> MTAI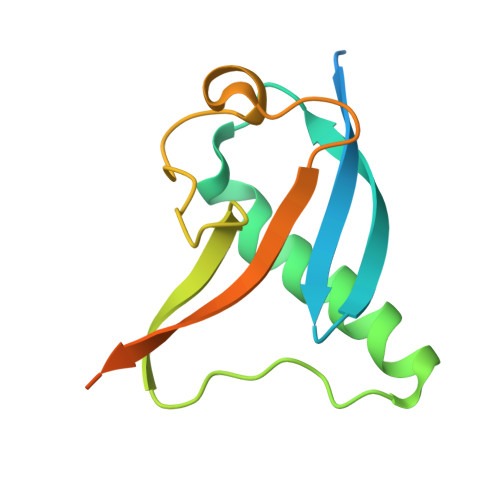VEAPQPGAEAIASPQAAVVAIMAADVQIAVVLDAHAPISVMIDPLLKVVNTRLRELGVAPLEAKGRGRWMLCLVDGTPLRPNLSLTEQEVYDGDRLWLKFLEDTEHRSEVIEHISTAVATNLSKR(pyren-1-yl)acetic acid | C18 H12 O2 | 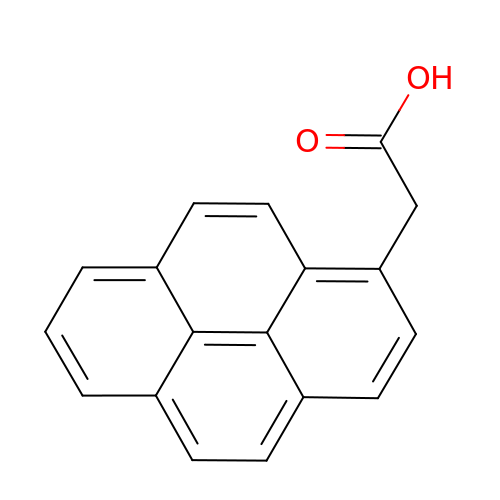SDJCLYBBPUHKCD-UHFFFAOYSA-N> GSHMKNSVSVDLPGSMKVLVSKSSNADGKYDLIATVDALELSGTSDKNNGSGVLEGVKADASKVKLTISDDLGQTTLEVFKSDGSTLVSKFVTSKDKSSTFEKFNE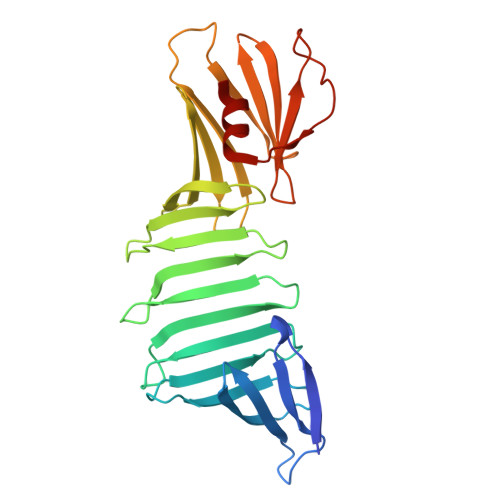KGEVSEKFITRADGTRLEYTGIKSDGSGKAKEVLKGYVLEGTLTAEKTTLVVKEGTVTLSKNISKSGEVSVELNDTDSSAATKKTAAWNSGTSTLTITVNSKKTKDLVFTSSNTITVQQYDSNGTSLEGSAVEITKLDEIKNALK>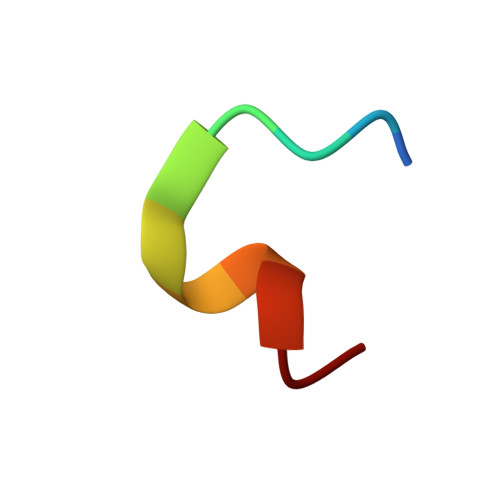 APIRYEWDEFC>MQYKKIITSESVGAGHPDKICDQISDAILDECLSQDQNSRVACEVLACNRLIVIAGEITTHAYVDVVKTAWEIIKPLGYDENDFTIISNVNKQSVDIAQSVDKTNKNLIGAGDQGIVFGYACDETPQYMPLTSVLAHELLKEIERQR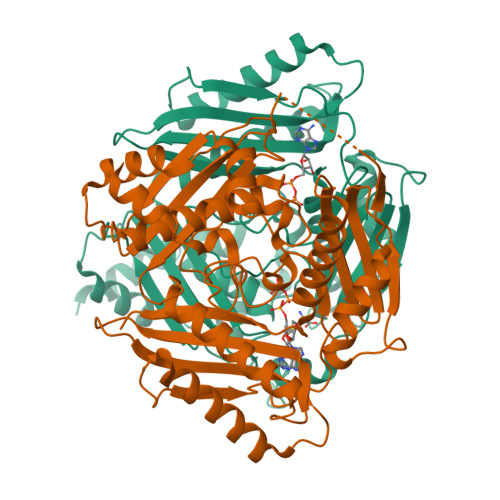RSKEFIKIQADMKSQVSIDYSNSTPLIETMLVSIQHDEDYDVEYFNKKVSAIMEQIAKKYNLNTNFKKIINSSGRFVIGGPIGDTGLTGRKIIVDTYGGVGHHGGGAFSGKDPTKVDRSASYFARWIAKNVVAAKLAKQCEIQLAFAIGQPQPVAMYVNTFNTNLIDETKIFEAIKKSFNFDIKTFINDLNLWTTKYLPVATYGHFGRDDLDLSWEKLNKVEDLIKNSKHHHHHH[4x]Diatoms rely on fucoxanthin chlorophyll a/c-binding proteins (FCPs) for their great success in oceans, which have a great diversity in their pigment, protein compositions, and subunit organizations. The light-harvesting antennas of the diatom PSII belong to the LHC family, but they bind Chl a/c instead of Chl a/b, and a large amount of fucoxanthin (Fx) instead of β-carotene (BCR), to harvest blue-green light; hence, they are called FCPs (fucoxanthin Chl a/c binding proteins). Lhcf proteins are the major antennas for PSII, whereas Lhcr proteins are mainly connected to PSI, and Lhcx proteins are considered to be mainly involved in photoprotection, as some of the Lhcx proteins have been found to function similarly to the LHCSR proteins in green algae. We report a unique structure of photosystem II (PSII)–FCPII supercomplex from Thalassiosira pseudonana at 2.68-Å resolution by cryo–electron microscopy.

The interactions within the Tp-Lhcf6-Lhcf11 heterodimer are similar to those in the Tp-Lhcf7 homodimer, such as interactions between the coupled helices C and Chls a406. Furthermore, LHG520 of Tp-Lhcf11 and LHG512 of Tp-Lhcf6 are inserted into the interface between the two monomers and strengthen their associations. Tp-Lhcf6 in the heterodimer has a longer AC-loop and a shorter C terminus than Tp-Lhcf11, which is unsuitable to interact with Tp-Lhca2. The long N terminus of Tp-Lhca2 and the AC-loop of Tp-Lhcf11 form tight, hydrophobic interactions at the stromal surface. In addition, a pair of hydrogen bond between Arg150 of Tp-Lhcf11 and Pro59 of Tp-Lhca2 and a large number of pigments and lipids contribute to the stable binding between Tp-Lhca2 and Tp-Lhcf11. (B) The long C terminus of Lhca2 extends to the PSII core and interacts with CP43, PsbW, D1, PsbQ, and PsbO at the luminal surface region. Tp-Lhcf5 was associated at the outside of Tp-Lhca2 loosely by its N- and C-terminal loops and has no direct interactions with Tp-Lhcf6. Both Tp-Lhcf5 and Tp-Lhcf6 are in the periphery of the supercomplex and rich in Fx; thus, they may harvest more green light. Owing to tight interactions between Tp-Lhcf11 and Tp-Lhca2, more efficient EET pathways are formed by Chl a410 of Tp-Lhcf11 to Chl a614 of Tp-Lhca2 (5.7 Å) and Chl a413 of Tp-Lhcf11 to Chl a612 of Tp-Lhca2 (8.8 Å). The shifted Chl a605 and extra Chl a613 of Tp-Lhca2 may receive energy from Chl a401 and Chl a402 of Tp-Lhcf5 at distances of around 8.0 Å; thus, energy captured by Lhcf5 is eventually transferred through Lhca2 to the PSII core.

> WNEAPRALPFGSAPPTLDGSLVGDVGFDPIGFSTAPFASFNNPIYQEGNFMTDVQWLREAELTHGRIAQLAVVGFIWPALFGTFPGNENFGGADAYSYVNPLEAINHIPSLAIYQIVGGMAWVEYQRVQRIKEQGKDRISGDIGLAYPGGWNPFNINYSPEEYAEKQLQEIKHCRLAMLGAFGLFFQALNSGEDIVSQLSPAFAAPEYAAKAGYFLPQGI;> ENEIGVLPPTGFFDPAGLSDGISQEKFDSYRLAELKHGRAAMLAVLGYVAPETYRFGYDLIPGELSTNDIPNGVAAIKAIPFGGWAQMIAFVGCVETYGWFTSPTGVLDLPDDILAKRQTAELQHGRLAMLAFLELIRHDSQNLAQPGFDGLDNLITGLPFLY;> ESEIGAQAPLGFWDPLGFLDRADQETFDRLRYVELKHGRIAQLAFVGNLITRAGYHLPGDISLGRAFADVPNGIAAINGPDAISTAALLQTLAFIGFLETRVMIDATGESQFRGDFRNGFDFGWDKQSPEWQTNKRAIELNQGRAAMMGILGLMMHEQVG;> FENELGAQPPLGFFDPLGMLDEAGQARFDRLRYVELKHGRICQLAFLGNIITRAGIHLPGAISLDGTKFSDIGNGWAGSFEVPKDGALQILFFVGFLELFVMKDVTGEGEFVGDFRNGALDFGWDSFSEETKLQKRAIELNNGRAAMMGILGLMVHEQLGGELPIVGQ>SGRGEAETRECIYYNANWELERTNQSGLERCEGEQDKRLHCYASWRNSSGTIELVKKGCWLDDFNCYDRQECVATEENPQVYFCCCEGNFCNERFTHLPEAGGPEVTYEPPPTAPTGGGTHTCPPCPAPELLG[2x];>TACRKHELYVSFQDLGWQDWIIAPKGYAANYCDGECSFPLNAHMNATNHAIVQTLVHLMNPEYVPKPCCAPTKLNAISVLYFDDNSNVILKKYRNMVVRACGCH[2x];>[2x]QNLDSMLHGTGMKSDLDQKKPENGVTLAPEDTLPFLKCYCSGHCPDDAINNTCITNGHCFAIIEEDDQGETTLASGCMKYEGSDFQCKDSPKAQLRRTIECCRTNLCNQYLQPTLPPVVIGPFFDGSIRDKTHTCPPCPAPELLG

ALK2 is a type I receptor that binds two different ligand classes of the BMP/TGF-β superfamily: the BMPs and the Activins. With BMP ligands, ALK2 signals to play roles in bone modeling, while with activins, ALK2 regulates signaling by forming nonsignaling complexes. To explore, at the molecular level, how ALK2 interacts with its cognate ligands, we utilized cryoelectron microscopy (cryoEM) to resolve the ternary complex structures of ALK2:ActRIIB:BMP6 and ALK3:ActRIIB:BMP6. The overall complex assembly of ligand:receptors is consistent with previous BMP complex structures, with the type II receptor binding at the convex, “knuckle” of the β-ribbons and the type I receptor binding at the interface built from the concave fold of the fingers and the wrist helix.

We used a similar experimental setup to resolve the structure of ALK3-ActRIIB bound to BMP6 to 3.3Å with residues, ALK3 (50 to 141), ActRIIB (26 to 117), and BMP6 mature domain (410 to 513), being well-resolved. During interaction with ALK3, BMP6 buries a total of ~1,325.4 Å2, similar to that of ALK3:BMP2 (25), while only burying 1,113.8 Å2 while engaging ALK2. Conversely, ALK3 caps the wrist helix with residue Gln117, engaging Asn469 of the posthelical loop of BMP6, whereas ALK2 does not. This interaction is facilitated by a three amino acid extension in the β4β5 loop of ALK3, not present in ALK2. Given the lack of direct binding between the carbohydrate moiety of BMP6 and ALK2, it remains curious why ALK2 is reliant on the presence of the carbohydrates for BMP6 binding, whereas ALK3 is not. Comparison between the CryoEM structure of ALK2:BMP6 and ALK3:BMP6 reveals the presence of a salt bridge between ALK3 residue Asp69 and BMP6 residue Arg413, which sterically occludes the previously mentioned His452 driven hydrophobic contacts in BMP6. We hypothesized that ALK3 utilizes this salt bridge to stabilize the prehelix loop without relying on the carbohydrate moiety. Conversely, deglycosylation of BMP6 does not reduce binding to ALK3-ActRIIB-Fc to the same degree (KD of 30.0 pM and 35.1 pM for BMP6 and dgBMP6, respectively). In contrast, BMP2 binding was similar between ALK3 and ALK3.D69G, where only introduction of the β1β2 from ALK2 reduces binding significantly. These data support that the salt bridge between ALK3 Asp69 and BMP6 Arg413 stabilizes binding and constitutes an alternative strategy to stabilize the prehelix loop in the absence of glycosylation. With ALK2, BMP6 utilizes a glycosylation on Asn454 to form interchain contacts that stabilize the prehelix in the active conformation, whereas with ALK3, BMP6 utilizes a salt bridge to stabilize the same interface.> SKRYFVTGTDTEVGKTV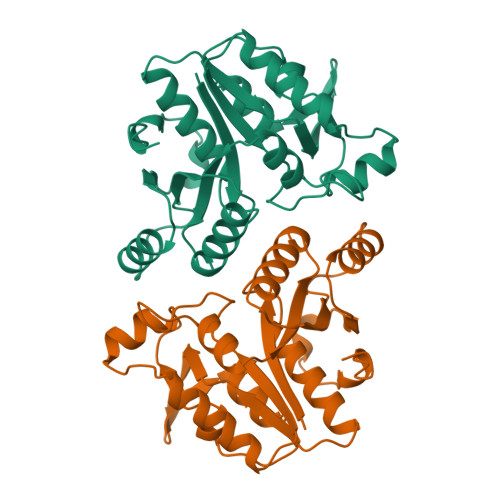ASCALLQAAKAAGYRTAGYKPVASGSEKTPEGLRNSDALALQRNSSLQLDYATVNPYTFAEPTSPHIISAQEGRPIESLVMSAGLRALEQQADWVLVEGAGGWFTPLSDTFTFADWVTQEQLPVILVVGVKLGCINHAMLTAQVIQHAGLTLAGWVANDVTPPGKRHAEYMTTLTRMIPAPLLGEIPWLAENPENAATGKYINLALL> K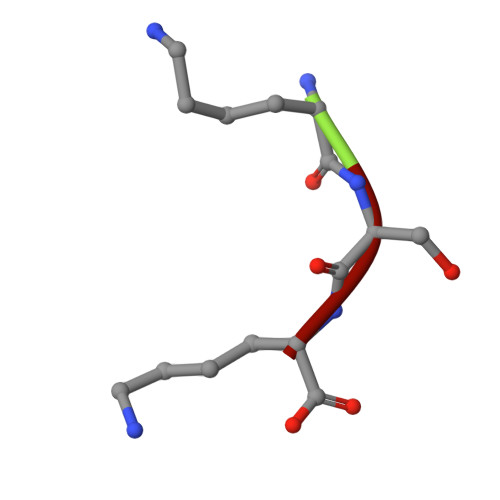SK2-(4-ethylsulfonylphenyl)-~{N}-[4-(2-phenylmethoxypyridin-3-yl)thiophen-2-yl]ethanamide | C26 H24 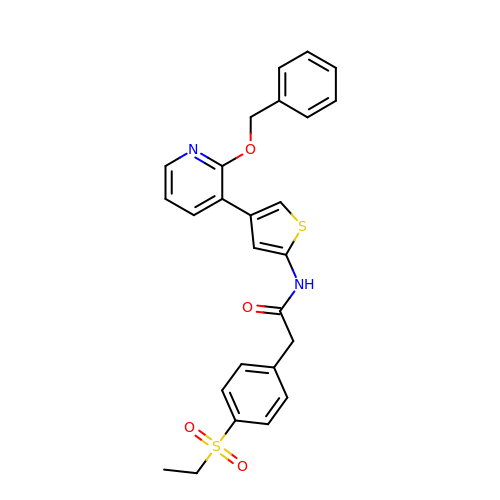N2 O4 S2 | RHPSXPWLHPRNOB-UHFFFAOYSA-N>[6x]MYEEFPDVITFQSYVEQSNGEGGKTYKWVDEFTAAAHVQPISQEEYYKAQQLQTPIGYNIYTPYDDRIDKKMRVIYRGKIVTFIGDPVDLSGLQEITRIKGKEDGAYVG;>[12x]MADIYPLGKTHTEELNEIIVESAKEIAEPDTTMIQKLIDEHNPEPLLKGVRYYMCENDIEKKRRTYYDAAGQQLVDDTKTNNRTSHAWHKLFVDQKTQYLVGEPVTFTSDNKTLLEYVNELADDDFDDILNETVKNMSNKGIEYWHPFVDEEGEFDYVIFPAEEMIVVYKDNTRRDILFALRYYSYKGIMGEETQKAELYTDTHVYYYEKIDGVYQMDYSYGENNPRPH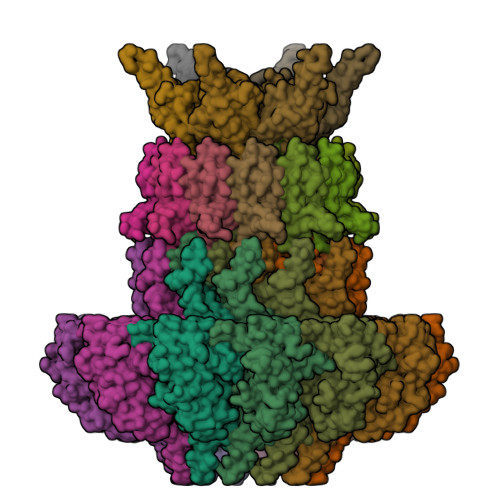MTKGGQAIGWGRVPIIPFKNNEEMVSDLKFYKDLIDNYDSITSSTMDSFSDFQQIVYVLKNYDGENPKEFTANLRYHSVIKVSGDGGVDTLRAEIPVDSAAKELERIQDELYKSAQAVDNSPETIGGGATGPALENLYALLDLKANMAERKIRAGLRLFFWFFAEYLRNTGKGDFNPDKELTMTFTRTRIQNDSEIVQSLVQGVTGGIMSKETAVARNPFVQDPEEELARIEEEMNQYAEMQGNLLDDEGGDDDLEEDDPNAGAAESGGAGQVS;>MDIQRVKRLLSITNDKHDEYLTEMVPLLVEFAKDECHNPFIDKDGNESIPSGVLIFVAKAAQFYMTNAGLTGRSMDTVSYNFATEIPSTILKKLNPYRKMAR[12x]>YVEFEPSDKHIK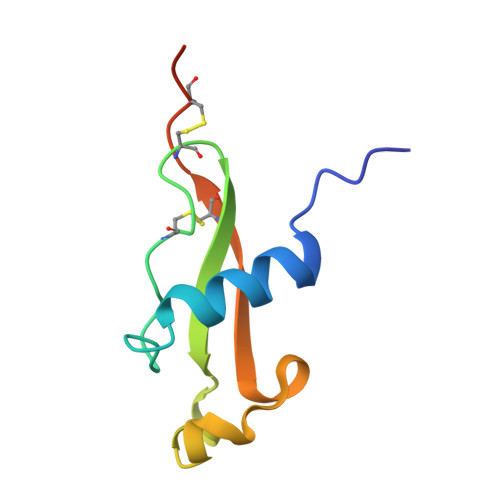EYLNKIQNSLSTEWSPCSVTCGNGIQVRIKPGSANKPKDELDYANDIEKKICKMEKCPHHHHHHA[3x]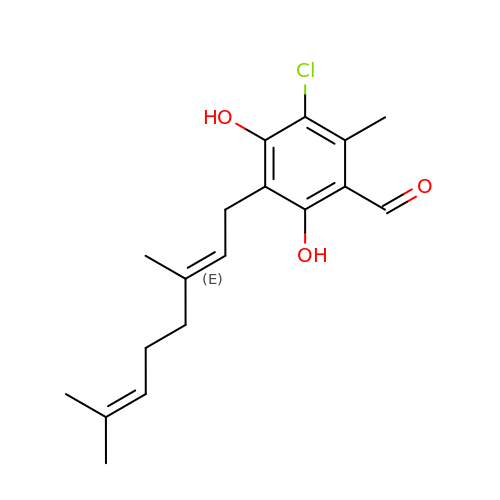3-chloro-5-[(2E)-3,7-dimethylocta-2,6-dien-1-yl]-4,6-dihydroxy-2-methylbenzaldehyde | C18 H23 Cl O3 | UEUMAXMCCDEOIJ-XYOKQWHBSA-N>MMDQARSAFSNLFGGEPLSYTRFSLARQVDGDNSHVEMKLAVDEEENADNNTKANVTKPKRCSGSICYGTIAVIVFFLIGFMIGYLGYCKGVEPKTECERLAGTESPVREEPGEDFPAARRLYWDDLKRKLSEKLDSTDFTGTIKLLNENSYVPREAGSQKDENLALYVENQFREFKLSKVWRDQHFVKIQVKDSAQNSVIIVDKNGRLVYLVENPGGYVAYSKAATVTGKLVHANFGTKKDFEDLYTPVNGSIVIVRAGKITFAEKVANAESLNAIGVLIYMDQTKFPIVNAELSFFGHAHLGTGDPYTPGFPSFNHTQFPPSRSSGLPNIPVQTISRAAAEKLFGNMEGDCPSDWKTDSTCRMVTSESKNVKLTVSNVLKEIKILNIFGVIKGFVEPDHYVVVGAQRDAWGPGAAKSGVGTALLLKLAQMFSDMVLKDGFQPSRSIIFASWSAGDFGSVGATEWLEGYLSSLHLKAFTYINLDKAVLGTSNFKVSASPLLYTLIEKTMQNVKHPVTGQFLYQDSNWASKVEKLTLDNAAFPFLAYSGIPAVSFCFCEDTDYPYLGTTMDTYKELIERIPELNKVARAAAEVAGQFVIKLTHDVELNLDYERYNSQLLSFVRDLNQYRADIKEMGLSLQWLYSARGDFFRATSRLTTDFGNAEKTDRFVMKKLNDRVMRVEYHFLSPYVSPKESPFRHVFWGSGSHTLPALLENLKLRKQNNGAFNETLFRNQLAL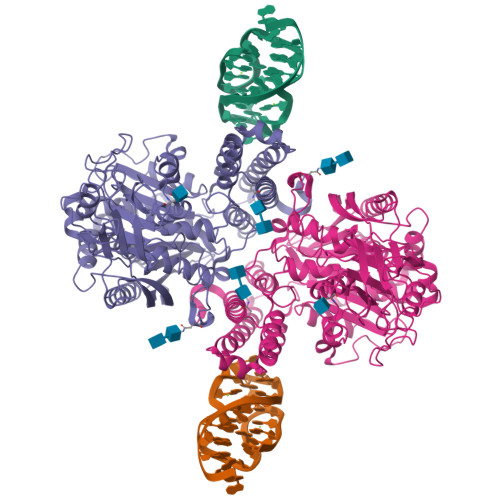ATWTIQGAANALSGDVWDIDNEF[2x]> SDRVRSITLGNSTITTQECANVVVGYGRWPTYLRDDEATAEDQPTQPDVATCRFYTLDSIKWEKGSVGWWWKFPEALSDMGLFGQNMQYHYLGRAGYTIHVQCNASKFHQGCLLVVCVPEAEMGGAVVGQAFSATAMANGDKAYEFTSAT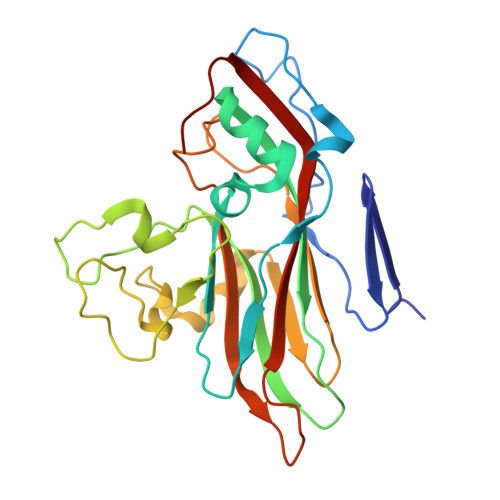QSDQTKVQTAIHNAGMGVGVGNLTIYPHQWINLRTNNSATIVMPYINSVPMDNMFRHYNFTLMVIPFVKLDYADTASTYVPITVTVAPMCAEYNGLRLAQAQ5'-O-[(S)-(cyclopentyloxy)(hydroxy)phosphoryl]adenosine | C15 H22 N5 O7 P | 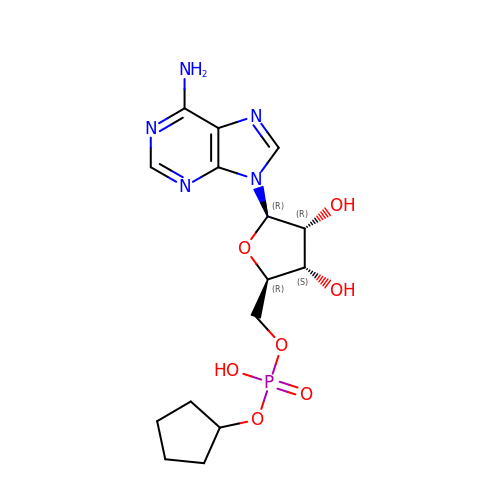ILDPDEYZUPQLBS-SDBHATRESA-N>TAPSQVLKIRRPDDWHLHLRDGDMLKTVVPYTSEIYGRAIVMPNLAPPVTTVEAAVAYRQRILDAVPAGHDFTPLMTCYLTDSLDPNELERGFNEGVFTAAKLYPANASTNSSHGVTSVDAIMPVLERMEKIGMPLLVHGEVTHADIDIFDREARFIESVMEPLRQRLTALKVVFEHITTKDAADYVRDGNERLAATITPQHLMFNRNHMLVGGVRPHLYCLPILKRNIHQQALRELVASGFNRVFLGTDSAPHARHRKESSCGCAG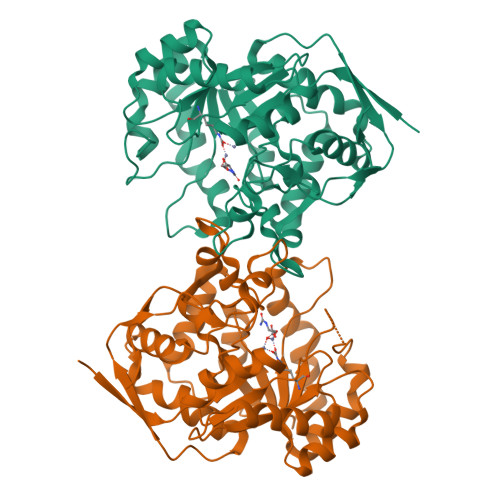CFNAPTALGSYATVFEEMNALQHFEAFCSVNGPQFYGLPVNDTFIELVREEQQVAESIALTDDTLVPFLAGETVRWSVKQ[2x]> MSAGINYVQNYNGNLGDFTYDESAGTFSMYWEDGVSSDFVVGLGWTTGSSNAITYSAEYSASGSSSYLAVYGWVNYPQAEYYIVEDYGDYNPCSSATSLGTVYSDGSTYQVCTDTRTNEPSITGTSTFTQYW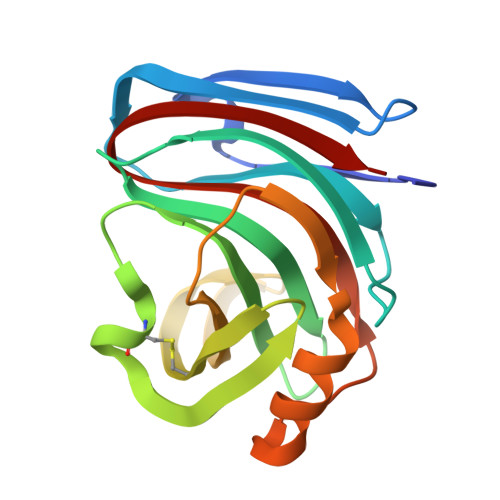SVRESTRTSGTVTVANHFNFWAQHGFGNSDFNYQVMAVEAWSGAGSASVTISS>[2x]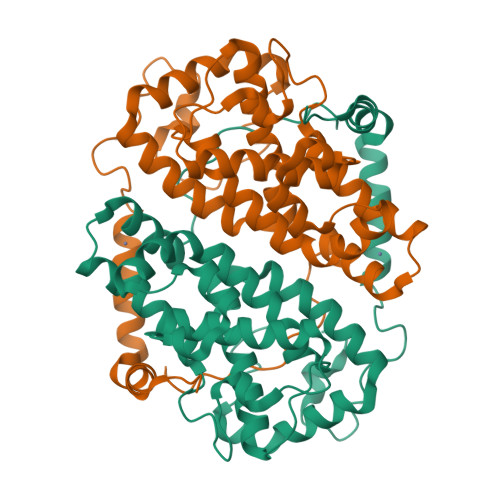GPGAADTIDATTRLVLRSISERAAVDRISESFGRSAQVMHDPFGGQPFPAANSPWAPVLAGQGGPFDAETRRVSWETLVAHGPSLYRTFAGNPRAASTAKAMRDCVLRQENFIEALASADETLAWCKMCIHHNLPLRPQDPIIGTTAAVLDNLATRLRPFLQCYLKARGLCGLDELCSRRRLADIKDIASFVFVILARLANRVERGVAEIDYATLGVGVGEKMHFYLPGACMAGLIEILDTHRQECSSRVCELTASHIVAPPYVHGKYFYCNSLF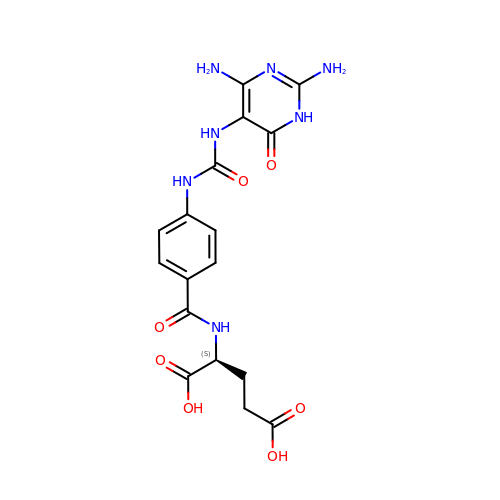(2S)-2-[[4-[[2,4-bis(azanyl)-6-oxidanylidene-1H-pyrimidin-5-yl]carbamoylamino]phenyl]carbonylamino]pentanedioic acid | C17 H19 N7 O7 | WBQDVZMETQWVQD-VIFPVBQESA-N>[6x]MAQDALSDGFVRLCIDPSLNFFG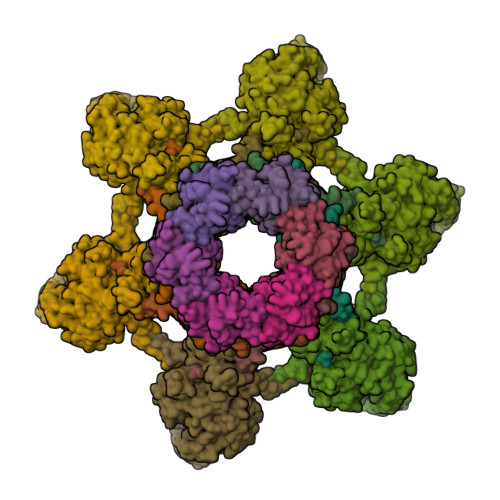EGCKILVEGQITDDATAAENVVTCVNSELDLVERFGQGSVLTESLRKVFCMCKSGVSVYALPRADAAAAVSAVYTLTVTGTALTDGRVQLYMGEAEYSLDIGVDEGDTPTQIAAKIVAAISPDFPYEATAAAGVITLTARNGGTIGNHLSVIYTNLGSCTSVTPEGVTVAFAQTTPGSVNPEPNDYASVVNECCFAVYVLSSDDTDWQENLRDWIRSAWDCSKPQCFGHGYVFNKGTLGQVLADGDNSAELSRLALPTTYPVLPYLTNAAYGALSACSTCENPELNVQGQTYGLLSCINMPESCTPGWEFTEVTQLQNNGFVVSGPATTSGQGNFTSPYIYNDVTNYLRDEKNRPNATFRDASSRRLAAATGVALATFLQQFNGLAVFTKNTNIKTGIIGTNLRLMLGKIRKWASDNVGVLFSEFDNINEDIQLVSDFDVQPKCVGQPGVFHLNMRYRPPVRGARINVNLVPALFDNCDR;>[6x]METKLKLTYSNRLTLPEIAKHIVSPTFHELEGRAIPVTGVEDDKEGQSAITKPFALVGLRIGDTSGPAEIGENSRINLRDDFIIEFNFNKDRYKKGGAETSLFSYYDYESIRDRLFNAMVAFAGEYGITFEFVSLDISTEGDTVYIEFRFRQNFDWCEADRESDTVIKAGSFSLNLKGC;>MACNKQNGVKNILITFTHCDTGEVIGPISHEQPDDTLPTYKTCAWTNTALTNGAVMRSASNATMTLPVVRDPRVPLAWYQGCAQIDAQVEKFDGTVMTLTEGAVTEPEESDGRAVTMTIIAAEIDELLPPGSLAAA[6x];>MKIKDRKHRVIVCSQKSDVDDNGQLLISRTGSINGWAAIEPVKAIRFSKDGVSMQKDTFQPTHDITMNYNPDVNISVSAWVYEHRLKSPPRWFKVISVINVDECSQFMRLRSRLVESNDEVEKPVSEENSFGAVKIDIPL[6x]Coupled binuclear copper (CBC) proteins contain a type-3 copper site that reversibly binds dioxygen. Tyrosinase catalyses o-hydroxylation of monophenols to o-diphenols (mono-oxygenase activity) and the subsequent oxidation of o-diphenols to the corresponding o-quinones (diphenolase activity). Catechol oxidase only catalyses the latter reaction, and o-aminophenol oxidase catalyses oxidation of o-aminophenols to o-quinoneimines in the grixazone biosynthetic pathway. The overall structure of AoCO4 shows a four-helix bundle around the copper-binding site, as seen in all CBC proteins. In AoCO4, His102, His110, His119 and His284, His288 and His312 are responsible for CuA and CuB binding, respectively.

Two new crystal structures, called met/deoxy (an average of met -and deoxy-forms) and deoxy, were solved at 1.8- and 2.5-Å resolutions, respectively. In this triclinic crystal form, the citrate ion forms crystal contacts between molecules A and B, resulting in symmetry with two homodimers in the asymmetric unit. In the met/deoxy structure, the copper sites of the A, B and D molecules were refined with one water molecule between CuA and CuB. In met/deoxy, one water molecule is refined between the copper ions in molecules A, B and D, but the distances from copper to water are relatively long (2.3–2.4 Å), and therefore it is not a typical met-form. The copper centre does not represent a fully reduced deoxy-form either because a clear electron density for one water molecule is obtained. The copper site has features of both met- and deoxy-forms and from this perspective, the copper centre is named as met/deoxy. In molecule C, a peroxide ion was refined between the copper ions. The Cu-Cu distances were 4.3, 4.4, 4.4 and 4.5 Å for molecules A, B, C and D, respectively. However, some signs of oxy-form are obtained at least in molecule C. We believe that met/deoxy structure is only partly reduced, and it represents predominantly a mixture of met- and deoxy-forms. Interestingly, the signs of general radiation damage, such as partial disulphide bond breakage, were only observed in the met/deoxy structure, probably due to the higher resolution.

>[4x]AATATLPTTASSSTAVASSQLDQLANFAYNVTTDSVAGGSESKRGGCTLQNLRVRRDWRAFSKTQKKDYINSVLCLQKLPSRTPAHLAPGARTRYDDFVATHINQTQIIHYTGTFLAWHRYFIYEFEQALRDECSYTGDYPYWNWGADADNMEKSQVFDGSETSMSGNGEYIPNQGDIKLLLGNYPAIDLPPGSGGGCVTSGPFKDYKLNLGPAALSLPGGNMTAAANPLTYNPRCMKRSLTTEILQRYNTFPKIVELILDSDDIWDFQMTMQGVPGSGSIGVHGGGHYSMGGDPGRDVYVSPGDTAFWLHHGMIDRVWWIWQNLDLRKRQNAISGTGTFMNNPASPNTTLDTVIDLGYANGGPIAMRDLMSTTAGPFCYVYL Defensins are a family of antimicrobial peptides of innate immunity broadly active against bacteria, viruses and toxins. They are small (2–5 kDa), stabilized structurally by three disulfide bonds, form oligomers, and are divided into α, β and θ structural classes. The canonical dimer interface of HNP1 is formed by the antiparallel extensions of the β2 strands stabilized by the reciprocal main-chain hydrogen bonds contributed by Thr18 and Ile20, and the hydrophobic packing of the side chains of Tyr16, Tyr21, Trp26, Phe28 and the Cys2–Cys30 and Cys4–Cys19 disulfides. Further analysis of probable quaternary structures by the Protein Interfaces, Surfaces and Assemblies (PISA) software indicates that the HNP1 dimer forms a tetramer or dimer of dimers in a crystal.

The dimer-dimer interface consists of the Ile20 and Leu25 side chains and the assembly is maintained exclusively through van der Waals interactions. Surprisingly, although the asymmetric unit of the I20A-HNP1 crystal contained two monomers they were not arranged into a dimer. Analysis of intermolecular contacts within the crystal unambiguously rules out the formation of any quaternary structure for the I20A-HNP1 mutant. In the present study, we also discovered novel quaternary structures in the crystal, including a form of I20A-HNP1 that appears to be unable to form dimers or tetramers and a novel tetrameric form of I20A/L25A-HNP1. The functional consequences of the I20A and L25A mutations, alone or in concert, were milder than the Y16A/F28A double mutant or the quadruple mutant. LF inhibition was less than 2-fold different than wild-type for the single mutants and about 2-fold different for the I20A/L25A double mutant, as measured by IC50 values. In the virtual colony count assay, whereas the I20A and L25A mutations each made a significant difference against S. aureus, they did not make a significant difference against E. coli or B. cereus even in the I20A/I25A double mutant. Since Ile20 and Leu25 function as an isologous binding site for the formation of a dimer of dimers, their effect or lack thereof on E. coli is not surprising, given a previous study of N-methylated Ile20 that showed that dimerization is dispensible for E. coli activity.

>[2x]ACYCRIPACIAGERRYGTCAYQGRLWAFCC>[5x]MNVIAILNHMGVYFKEEPIRELHRALERLNFQIVYPNDRDDLLKLIENNARLCGVIFDWDKYNLELCEEISKMNENLPLYAFANTYSTLDVSLNDLRLQISFFEYALGAAEDIANKIKQTTDEYINTILPPLTKALFKYVREGKYTFCTPGHMGGT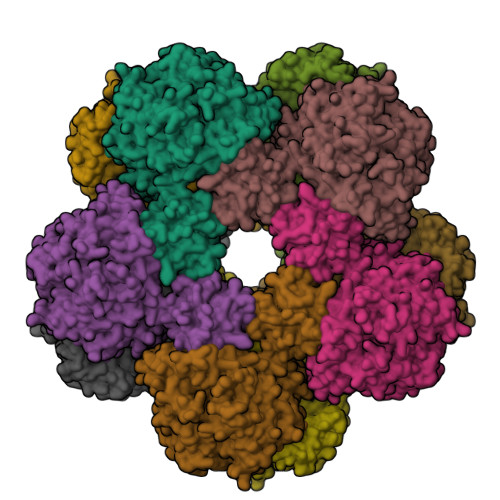AFQKSPVGSLFYDFFGPNTMKSDISISVSELGSLLDHSGPHKEAEQYIARVFNADRSYMVTNGTSTANKIVGMYSAPAGSTILIDRNCHKSLTHLMMMSDVTPIYFRPTRNAYGILGGIPQSEFQHATIAKRVKETPNATWPVHAVITNSTYDGLLYNTDFIKKTLDVKSIHFDSAWVPYTNFSPIYEGKCGMSGGRVEGKVIYETQSTHKLLAAFSQASMIHVKGDVNEETFNEAYMMHTTTSPHYGIVASTETAAAMMKGNAGKRLINGSIERAIKFRKEIKRLRTESDGWFFDVWQPDHIDTTECWPLRSDSTWHGFKNIDNEHMYLDPIKVTLLTPGMEKDGTMSDFGIPASIVAKYLDEHGIVVEKTGPYNLLFLFSIGIDKTKALSLLRALTDFKRAFDLNLRVKNMLPSLYREDPEFYENMRIQELAQNIHKLIVHHNLPDLMYRAFEVLPTMVMTPYAAFQKELHGMTEEVYLDEMVGRINANMILPYPPGVPLVMPGEMITEESRPVLEFLQMLCEIGAHYPGFETDIHGAYRQADGRYTVKVLKEESKK>[3x]MSQVQFSHNPLFCIDIIKTYKPDFTPRVAFILGSGLGALADQIENAVAISYEKLPGFPVSTVHGHAGELVLGHLQGVPVVCMKGRGHFYEGRGMTIMTDAIRTFKLLGCELLFCTNAAGSLRPEVGAGSLVALKDHINTMPGTPMVGLNDDRFGERFFSLANAYDAEYRALLQKVAKEEGFPLTEGVFVSYPGPNFETAAEIRMMQIIGGDVVGMSVV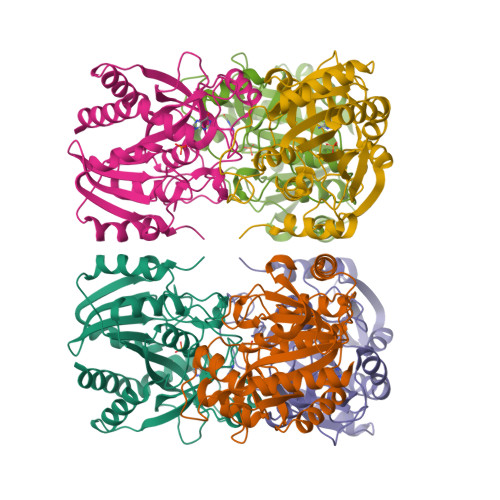PEVISARHCDLKVVAVSAITNMAEGLSDVKLSHAQTLAAAELSKQNFINLICGFLRKIA>MDCIFIFRRDLRLEDNTGLNYALSECDRVIPVFIADPRQLINNPYKSEFAVSFMINSLLELDDELRKKGSRLNVFFGEAEKVVSRFFNKVDAIYVNEDYTPFSISRDEKIRKVCEENGIEFKAYEDYLLTPKSLFHHRNFTSFYNEVSKVKVREPETMEGSFDVTDSSMNVDFLLTFKKIESPLFRGGRREGLYLLHRNVDFRRRDYPAENNNYRLSPHLKFGTISMREAYYTQKGKEEFVRELYWRDFFTLLAYYNPHVFGHCYRREYDNISWENNESYFEAWKEGRTGYPIIDAGMRMLNSTGYINGRVRMLVAFFLVKVLFVDWRWGERYFATKLVDYDPAINNGNWQWIASTGVDYMFRVFNPWKQQEKFDPEAKFIKEWVEELKDVPPSIIHSIYKTKVPGYPSPIVNWLERVNYVKSEYKNVKAVLLEHHHHHH[4x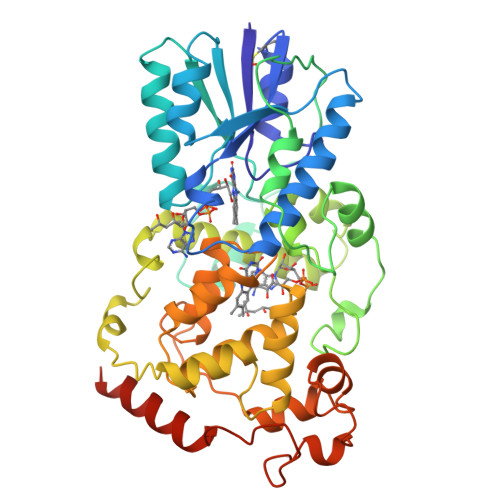]The P. falciparum protein PfEMP1(P. falciparum Erythrocyte Membrane Protein 1), expressed on the surface of IEs in a mutually exclusive manner, is responsible for the sequestration of IEs in various organs. It has been well established that in the case of PM, the PfEMP1 member VAR2CSA binds to low sulfated chondroitin sulfate A (CSA) or chondroitin sulfate proteoglycan (CSPG) expressed on placental intervillous tissue to mediate sequestration of IEs in the placenta. VAR2CSA is a >310 kDa protein comprising of multiple Duffy binding-like (DBL) domains and interdomains (ID) and shows specific and a higher binding affinity to CSA when compared with individual DBL and ID domains. Human pentameric immunoglobulin M (IgM) binds to several types of PfEMP1, including VAR2CSA via its Fc domain. Human pentameric IgM in a low resolution cryo-AFM study revealed mushroom-shaped architecture that consists of 5 copies of monomeric IgM and a J chain (JC).

In order to understand this observation, we used cryo-EM to derive a 3.6 Å map of an IgM-VAR2CSA complex, which reveals that IgM is sandwiched between two molecules of VAR2CSA. Our structure also shows that DBL3X and DBL5ε directly interact with the Cµ4 of IgM, possibly leading to the steric hinderance in VAR2CSA interaction with its receptor. Further from the overall view of the interacting surface, we observed interaction between chains E, G and K of IgM with I chain of VAR2CSA and chains F, D and B chain of IgM with M chain of VAR2CSA. Also, chain E of IgM interacts with DBL3x, chain G of IgM interacts with both DBL3x and DBL5ε and chain K of IgM interacts with DBL5ε. Similarly, chain F of IgM interacts with DBL3x, chain D of IgM with DBL3x and DBL5ε and B of IgM with DBL5ε, suggesting very similar interactions on both faces. Further, when we analyzed buried surface area using PDBePISA both VAR2CSA and IgM junction have a total buried surface area of ~1350 Å2 on each face, further suggesting similar interfaces. We observed that although they have an overall RMSD of 1.367 Å, both structures align well between the ID2 to ID3 domain but have major changes and movement of corresponding residues in the DBL5ε domain. However, Ala2280 that is distant from the interacting surface showed a large movement of 55.8 Å away from ID3, reflecting the huge shifts in the C-terminal domains of VAR2CSA and also suggesting that the regions away from IgM shift more than the region that are closer to the interfacing surface. This results in the formation of a closed architecture in C-terminus of VAR2CSA in the IgMVAR2CSA map that differs from the apo-VAR2CSA architecture. The clockwise and anti-clockwise rotation of the two VAR2CSA molecules on opposite faces of IgM juxtaposes C-termini of both VAR2CSA near the J chain, where IgM creates a wall between both VAR2CSA molecules and hinders its interaction with its receptor.

>[10x]GSASAPTLFPLVSCENSPSDTSSVAVGCLAQDFLPDSITFSWKYKNNSDISSTRGFPSVLRGGKYAATSQVLLPSKDVMQGTDEHVVCKVQHPNGNKEKNVPLPVIAELPPKVSVFVPPRDGFFGNPRKSKLICQATGFSPRQIQVSWLREGKQVGSGVTTDQVQAEAKESGPTTYKVTSTLTIKESDWLGQSMFTCRVDHRGLTFQQNASSMCVPDQDTAIRVFAIPPSFASIFLTKSTKLTCLVTDLTTYDSVTISWTRQNGEAVKTHTNISESHPNATFSAVGEASICEDDWNSGERFTCTVTHTDLPSPLKQTISRPKGVALHRPDVYLLPPAREQLNLRESATITCLVTGFSPADVFVQWMQRGQPLSPEKYVTSAPMPEPQAPGRYFAHSILTVSEEEWNTGETYTCVVAHEALPNRVTERTVDKSTGKPTLYNVSLVMSDTAGTCY;>[2x]MDSTSTIANKIEEYLGAKSDDSKIDELLKADPSEVEYYRSGGDGDYLKNNICKITVNHSDSGKYDPCEKKLPPYDDNDQWKCQQNSSDGSGKPENICVPPRRERLCTYNLENLKFDKIRDNNAFLADVLLTARNEGEKIVQNHPDTNSSNVCNALERSFADLADIIRGTDQWKGTNSNLEKNLKQMFAKIRENDKVLQDKYPKDQKYTKLREAWWNANRQKVWEVITCGARSNDLLIKRGWRTSGKSDRKKNFELCRKCGHYEKEVPTKLDYVPQFLRWLTEWIEDFYREKQNLIDDMERHREECTREDHKSKEGTSYCSTCKDKCKKYCECVKKWKTEWENQENKYKDLYEQNKNKTSQKNTSRYDDYVKDFFEKLEANYSSLENYIKGDPYFAEYATKLSFILNPSDANNPSGETANHNDEACNCNESGISSVGQAQTSGPSSNKTCITHSSIKTNKKKECKDVKLGVRENDKDLKICVIEDTSLSGVDNCCCQDLLGILQENCSDNKRGSSSNDSCDNKNQDECQKKLEKVFASLTNGYKCDKCKSGTSRSKKKWIWKKSSGNEEGLQEEYANTIGLPPRTQSLYLGNLPKLENVCEDVKDINFDTKEKFLAGCLIVSFHEGKNLKKRYPQNKNSGNKENLCKALEYSFADYGDLIKGTSIWDNEYTKDLELNLQNNFGKLFGKYIKKNNTAEQDTSYSSLDELRESWWNTNKKYIWTAMKHGAEMNITTCNADGSVTGSGSSCDDIPTIDLIPQYLRFLQEWVENFCEQRQAKVKDVITNCKSCKESGNKCKTECKTKCKDECEKYKKFIEACGTAGGGIGTAGSPWSKRWDQIYKRYSKHIEDAKRNRKAGTKNCGTSSTTNAAASTDENKCVQSDIDSFFKHLIDIGLTTPSSYLSNVLDDNICGADKAPWTTYTTYTTTEKCNKERDKSKSQSSDTLVVVNVPSPLGNTPYRYKYACQCKIPTNEETCDDRKEYMNQWSCGSARTMKRGYKNDNYELCKYNGVDVKPTTVRSNSSKLDGNDVTFFNLFEQWNKEIQYQIEQYMTNANISCIDEKEVLDSVSDEGTPKVRGGYEDGRNNNTDQGTNCKEKCKCYKLWIEKINDQWGKQKDNYNKFRSKQIYDANKGSQNKKVVSLSNFLFFSCWEEYIQKYFNGDWSKIKNIGSDTFEFLIKKCGNNSAHGEEIFSEKLKNAEKKCKENESTDTNINKSETSCDLNATNYIRGCQSKTYDGKIFPGKGGEKQWICKDTIIHGDTNGACIPPRTQNLCVGELWDKSYGGRSNIKNDTKELLKEKIKNAIHKETELLYEYHDTGTAIISKNDKKGQKGKNDPNGLPKGFCHAVQRSFIDYKNMILGTSVNIYEHIGKLQEDIKKIIEKGTPQQKDKIGGVGSSTENVNAWWKGIEREMWDAVRCAITKINKKNNNSIFNGDECGVSPPTGNDEDQSVSWFKEWGEQFCIERLRYEQNIREACTINGKNEKKCINSKSGQGDKIQGACKRKCEKYKKYISEKKQEWDKQKTKYENKYVGKSASDLLKENYPECISANFDFIFNDNIEYKTYYPYGDYSSICSCEQVKYYKYNNAEKKNNKSLCYEKDNDMTWSKKYIKKLENGRSLEGVYVPPRRQQLCLYELFPIIIKNEEGMEKAKEELLETLQIVAEREAYYLWKQYNPTGKGIDDANKKACCAIRGSFYDLEDIIKGNDLVHDEYTKYIDSKLNEIFGSSNTNDIDTKRARTDWWENETITNGTDRKTIRQLVWDAMQSGVRYAVEEKNENFPLCMGVEHIGIAKPQFIRWLEEWTNEFCEKYTKYFEDMKSKCDPPKRADTCGDNSNIECKKACANYTNWLNPKRIEWNGMSNYYNKIYRKSNKESEDGKDYSMIMAPTVIDYLNKRCHGEINGNYICCSCKNIGAYNTTSGTVNKKLQKKETECEEEKGPLDLMNEVLNKMDKKYSAHKMKCTEVYLEHVEEQLNEIDNAIKDYKLYPLDRCFDDQTKMKVCDLIADAIGCKDKTKLDELDEWNDMDLRGTYNKHKGVLIPPRRRQLCFSRIVRGPANLRSLNEFKEEILKGAQSEGKFLGNYYKEHKDKEKALEAMKNSFYDYEDIIKGTDMLTNIEFKDIKIKLDRLLEKETNNTKKAEDWWKTNKKSIWNAMLCGYKKSGNKIIDPSWCTIPTTETPPQFLRWIKEWGTNVCIQKQEHKEYVKSKCSNVTNLGAQASESNNCTSEIKKYQEWSRKRSIQWETISKRYKKYKRMDILKDVKEPDANTYLREHCSKCPCGFNDMEEMNNNEDNEKEAFKQIKEQVKIPAELEDVIYRIKHHEYDKGNDYICNKYKNIHDRMKKNNGNFVTDNFVKKSWEISNGVLIPPRRKNLFLYIDPSKICEYKKDPKLFKDFIYWSAFTEVERLKKAYGGARAKVVHAMKYSFTDIGSIIKGDDMMEKNSSDKIGKILGDTDGQNEKRKKWWDMNKYHIWESMLCGYREAEGDTETNENCRFPDIESVPQFLRWFQEWSENFCDRRQKLYDKLNSECISAECTNGSVDNSKCTHACVNYKNYILTKKTEYEIQTNKYDNEFKNKNSNDKDAPDYLKEKCNDNKCECLNKHIDDKNKTWKNPYETLEDTFKSKCDCPKPLPSPIKPDDLPPQADEPFLESRGPFEGKPIPNPLLGLDSTRTGHHHHHH;> EDERIVLVDNKCKCARITSRIIRSSEDPNEDIVERNIRIIVPLNNRENISDPTSPLRTRFVYHLSDLCKKCDPTEVELDNQIVTATQSNICDEDSATETCYTYDRNKCYTAVVPLVYGGETKMVETALTPDACYPD>GALKRAEELKTQANDYFKAKDYENAIKFYSQAIELNPSNAIYYGNRSLAYLRTECYGYALGDATRAIELDKKYIKGYYRRAASNMALGKFRAALRDYETVVKVKPHDKDAKMKYQECNKIVKQKAFERAIAGDEHKRSVVDSLDIESMTIEDEYSGPKLEDGKVTISFMKELMQWYKDQKKLHRKCAYQILVQVKEVLSKLSTLVETTLKETEKITVCGDTHGQFYDLLNIFELNGLPSETNPYIFNGDFVDRGSFSVEVILTLFGFKLLYPDHFHLLRGNHETDNMNQIYGFEGEVKAKYTAQMYELFSEVFEWLPLAQCINGKVLIMHGGLFSEDGVTLDDIRKIERNRQPPDSGPMCDLLWSDPQPQNGRSISKRGVSCQFGPDVTKAFLEENNLDYIIRSHEVKAEGYEVAHGGRCVTVFSAPNYCDQMGNKASYIHLQ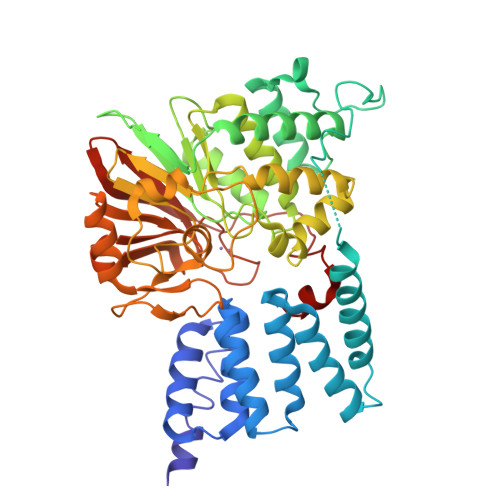GSDLRPQFHQFTAVPHPNVKPMAYANTLLQLGMM[4x]> MPEITRRRALTAAAAVAATASAAVTLAAPAASAAGHHEPAAPESFDEVYKGRRIQGRPAGGGAHHHEHGGGYEVFVDGVQLQVMRNADGSWIS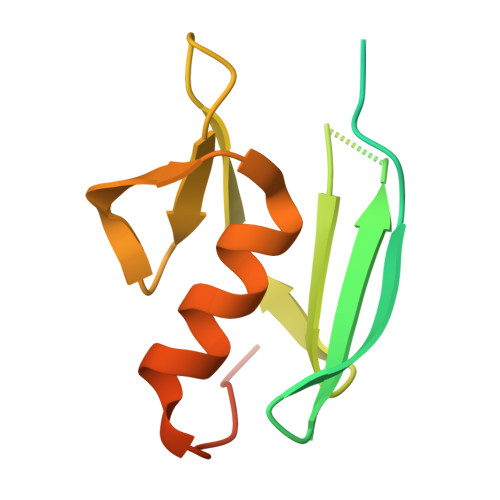VVSHYDPVPTPRAAARAAVDELQGAPLLPFPANLEHHHHHH> GMEEINKYIQNSSETGGEIYNLIEELFPICRSITGNGVRKTMDIIRKHIPLEIHEVKSGTKVFDWTVPKEWNIKDAYVRNSKGEKVIDFKENNLHVMSYSVPVHKTMTLDELKPYLHTIPGNKDRIPYLTSYYKENWGFSLTQNKFDELCDDDYEVVIDSSLEDGSLTYGEYYIRGELEEEILLTTYTCHPSMCNDNLSGVALITFIAKALSKLKTKYSYRFLFAPETIGSITWLSRNEDKLKNIKMGLVATCVGDAGIKNYKRTKFGDAEIDKIVEKVLMHCGSEYYVADFFPWGSDERQF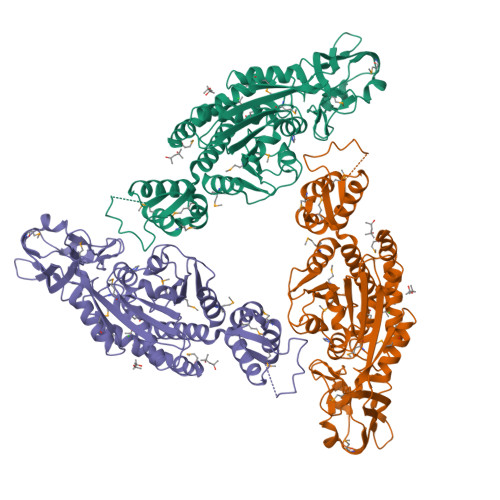SSPGINLSVGSLMRSCYGFDGYHTSADNLCYMNKDGLADSYKTYLEVIYTIENNRTYLNLNPKCEPQLGKRGIYRMIGGGSDYPFDEFAMFWVLNMSDGKNSLLDIAYKSGMEFRRIKYAADALYRVELLKLV>[8x]MAIERTLSIVKPDAVSKNHIGEIFARFEKAGLKIVATKMKHLSQADAEGFYAEHKERGFFGDLVAF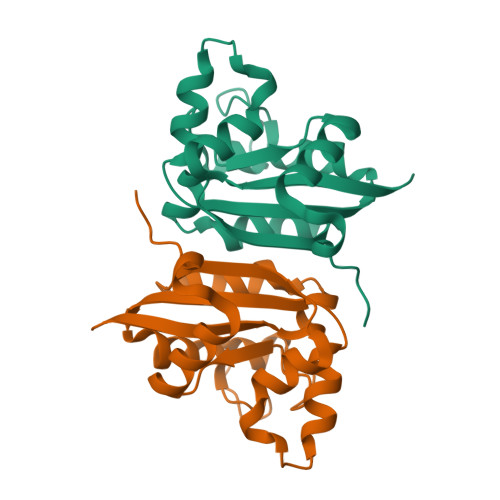MTSGPVVVSVLEGENAVLAHREILGATNPKEAAPGTIRADFAVSIDENAAHGSDSVASAEREIAYFFADNEICPRTR> MHHHHHHHDGTENPIHDRTSDYHKYLKVKQGDSDLFKLTVSDKRYIWYNPDPKERDSYECGEIVSETSDSFTFKTVDGQDRQVKKDDANQRNPIKFDGVEDMSELSYLNEPAVFHNLRVRYNQDLIYTYSGLFLVAVNPFKRIPIYTQEMVDIFKGRRRNEVAPHIFAISDVAYRSMLDDRQNQSLLITGESGAGKTENTKKVIQYLASVAGRNQANGSGVLEQQILQANPILEAFGNAKTTRNNNSSRFGKFIEIQFNSAGFISGASIQSYLLEKSRVVFQSETERNYHIFYQLLAGATAEEKKALHLAGPESFNYLNQSGCVDIKGVSDSEEFKITRQAMDIVGFSQEEQMSIFKIIAGILHLGNIKFEKGAGEGAVLKDKTALNAASTVFGVNPSVLEKALMEPRILAGRDLVAQHLNVEKSSSSRDALVKALYGRLFLWLVKKINNVLCQERKAYFIGVLDISGFEIFKVNSFEQLCINYTNEKLQQFFNHHMFKLEQEEYLKEKINWTFIDFGLDSQATIDLIDGRQPPGILALLDEQSVFPNATDNTLITKLHSHFSKKNAKYEEPRFSKTEFGVTHYAGQVMYEIQDWLEKNKDPLQQDLELCFKDSSDNVVTKLFNDPNIASRAKKGANFITVAAQYKEQLASLMATLETTNPHFVRCIIPNNKQLPAKLEDKVVLDQLRCNGVLEGIRITRKGFPNRIIYADFVKRYYLLAPNVP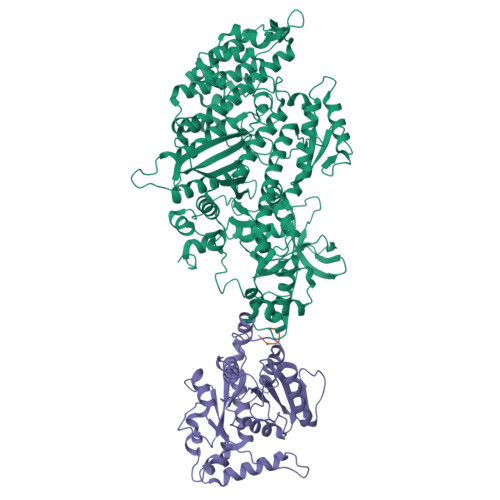RDAEDSQKATDAVLKHLNIDPEQYRFGITKIFFRAGQLARIEEAREQRISEI;> MEDLIPLVNRLQDAFSAIGQNADLDLPQIAVVGGQSAGKSSVLENFVGRDFLPRGSGIVTRRPLVLQLVNSTTEYAEFLHCKGKKFTDFEEVRLEIEAETDRVTGTNKGISPVPINLRVYSPHVLNLTLVDLPGMTKVPVGDQPPDIEFQIRDMLMQFVTKENCLILAVSPANSDLANSDALKIAKEVDPQGQRTIGVITKLDLMDEGTDARDVLENKLLPLRRGYIGVVNRSQKDIDGKKDITAALAAERKFFLSHPSYRHLADRMGTPYLQKVLNQQLTNHIRDTLPGLRNKLQSQL;> TRLVPRGSELALE> DDHSELLVNTKSGKVMGTRVPVLSSHISAFLGIPFAEPPVGNMRFRRPEPKKPWSGV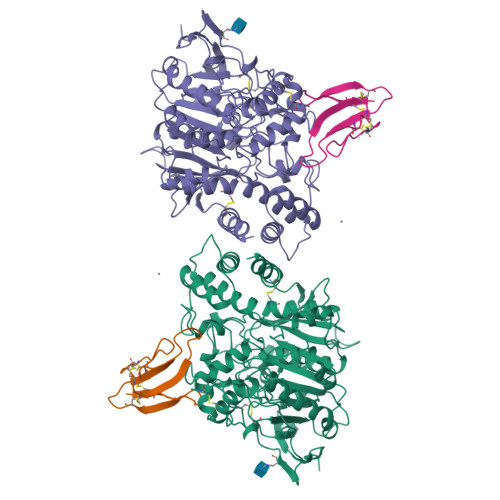WNASTYPNNCQQYVDEQFPGFSGSEMWNPNREMSEDCLYLNIWVPSPRPKSTTVMVWIYGGGFYSGSSTLDVYNGKYLAYTEEVVLVSLSYRVGAFGFLALHGSQEAPGNVGLLDQRMALQWVHDNIQFFGGDPKTVTIFGESAGGASVGMHILSPGSRDLFRRAILQSGSPNCPWASVSVAEGRRRAVELGRNLNCNLNSDEELIHCLREKKPQELIDVEWNVLPFDSIFRFSFVPVIDGEFFPTSLESMLNSGNFKKTQILLGVNKDEGSFFLLYGAPGFSKDSESKISREDFMSGVKLSVPHANDLGLDAVTLQYTDWMDDNNGIKNRDGLDDIVGDHNVICPLMHFVNKYTKFGNGTYLYFFNHRASNLVWPEWMGVIHGYEIEFVFGLPLVKELNYTAEEEALSRRIMHYWATFAKTGNPNEPHSQESKWPLFTTKEQKFIDLNTEPMKVHQRLRVQMCVFWNQFLPKLLNATAC;> TMCYSHTTTSRAILTNCGENSCYRKSRRHPPKMVLGRGCGCPPGDDNLEVKCCTSPDKCNY> TLLNPYFGEFGGMYVPQILMPALNQLEEAFVSAQKDPEFQAQFADLLKNYAGRPTALTKCQNITAGTRTTLYLKREDLLHGGAHKTNQVLGQALLAKRMGKSEIIAETGAGQHGVASALASALLGLKCRIYMGAKDVERQSPNVFRMRLMGAEVIPVHSGSATLKDACNEALRDWSGSYETAHYMLGTAAGPHPYPTIVREFQRMIGEETKAQILDKEGRLPDA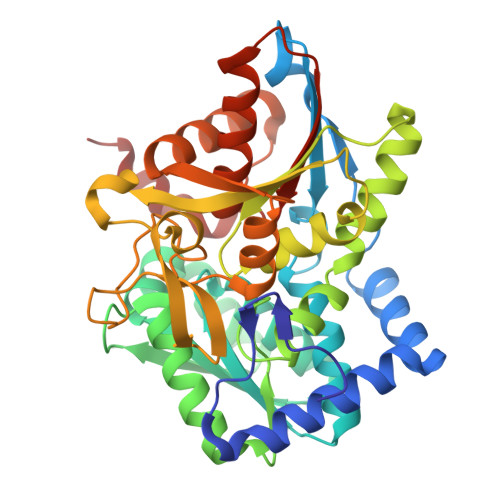VIACVGGGSNAIGMFADFINDTSVGLIGVEPGGHGIETGEHGAPLKHGRVGIYFGMKAPMMQTADGQIEESYSISAGLDFPSVGPQHAYLNSIGRADYVSITDDEALEAFKTLCRHEGIIPALESSHALAHALKMMREQPEKEQLLVVNLSGRGDKDIFTVHDILKA> TRPIDGLTDEDIREILTRYKKIALVGASPKPERDANIVMKYLLEHGYDVYPVNPNYEEVLGRKCYPSVLDIPDKIEVVDLFVDPAKAWRFVVYAIKKGAKVVWFQYNTYYPLAARQAKEAGLIIVANRCMMRE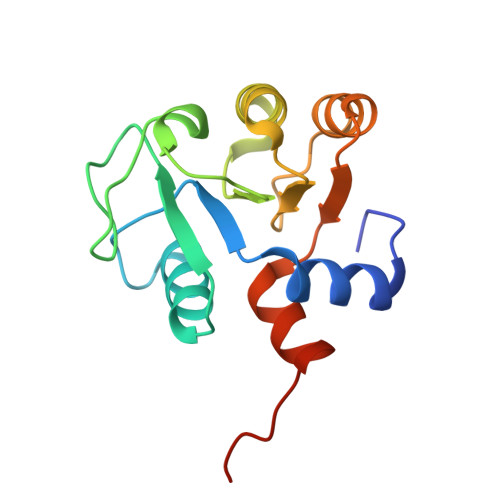HERLLGEKLEHHHHHH> CLAEGTRIFDPVTGTTHRIEDVVDGRKPIHVVAAAKDG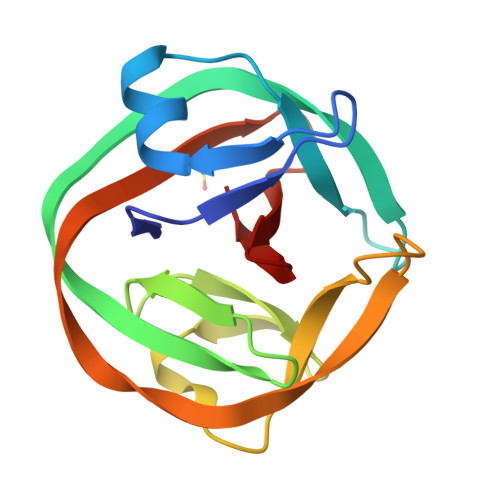TLHARPVVSWFDQGTRDVIGLRIAGGAIVWATPDHKVLTEYGWRAAGELRKGDRVAVRDVETGELRYSVIREVLPTRRARTFDLEVEELHTLVAEGVVVHN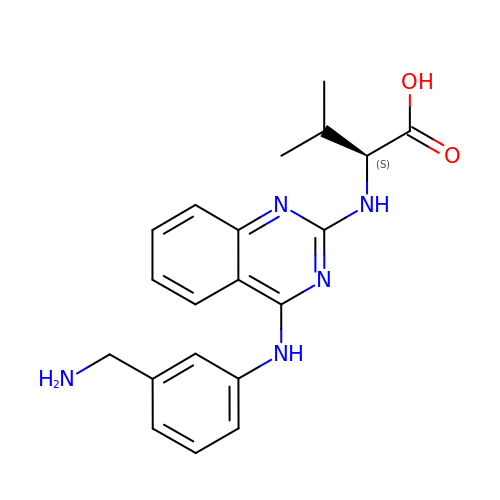(2~{S})-2-[[4-[[3-(aminomethyl)phenyl]amino]quinazolin-2-yl]amino]-3-methyl-butanoic acid | C20 H23 N5 O2 | SBAJWMCMBZQORT-KRWDZBQOSA-N>[2x]MGGKMEKITCVGHTALDYIFNVEKFPEPNTSIQIPSARKYYGGAAANTAVGIKKLGVNSELLSCVGYDFKNSGYERYLKNLDINISKLYYSEEEETPKAWIFTDKDNNQITFFLWGAAKHYKELNPPNFNTEIVHIATGDPEFNLKCAKKAYGNNLVSFDPGQDLPQYSKEMLLEI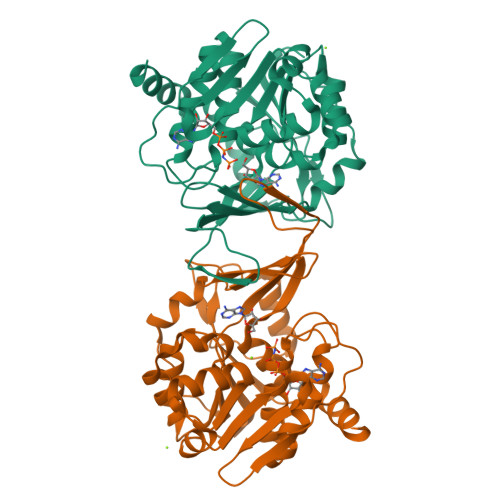IEHTNFLFMNKHEFERASNLLNFEIDDYLERVDALIVTKGSKGSVIYTKDKKIEIPCIKAGKVIDPTGAGDSYRAGFLSAYVKGYDLEKCGLIGAATASFVVEAKGCQTNLPTWDKVVERLEKHRI4-amino-N-[4-(benzyloxy)phenyl]butanamide | C17 H20 N2 O2 | 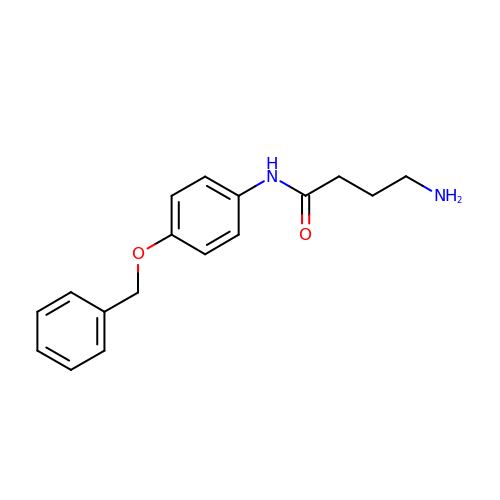QTWBKNVNGVYTNZ-UHFFFAOYSA-N>[2x]GAMGFFPSTEEEKQADKAIKDIENLIGESGFPELIENVCSLKH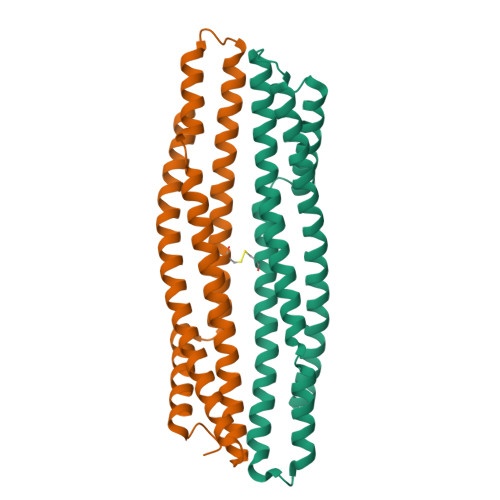EYTLIRSDFYDVITKIQNKKISLMKNSHNNRNKIRELVQLQNNLKIGDELDKIMGCIDTAEQEIRSAAFFFDEAKESLKEGIIKRLEKSKNRAASQLSKKALNRAEDALRCLENYSSKKGEAIGRRSFIKEVVEQAKNALSKS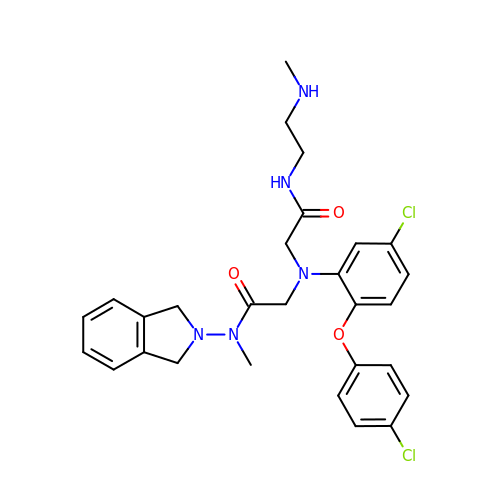2-{[5-chloro-2-(4-chlorophenoxy)phenyl](2-{[2-(methylamino)ethyl]amino}-2-oxoethyl)amino}-N-(1,3-dihydro-2H-isoindol-2-yl)-N-methylacetamide | C28 H31 Cl2 N5 O3 | AOQCCSFIEWPXMC-UHFFFAOYSA-N>[4x]GAMGSMATRIAILGAGPSGMAQLRAFQSAQEKGAEIPELVCFEKQADWGGQWNYTWRTGLDENGEPVHSSMYRYLWSNGPKECLEFADYTFDEHFGKPIASYPPREVLWDYIKGRVEKAGVRKYIRFNTAVRHVEFNEDSQTFTVTVQDHTTDTIYSAAFDYVVCCTGHFSTPYVPEFEGFEKFGGRILHAHDFRDALEFKDKTVLLVGSSYSAEDIGSQCYKYGAKKLISC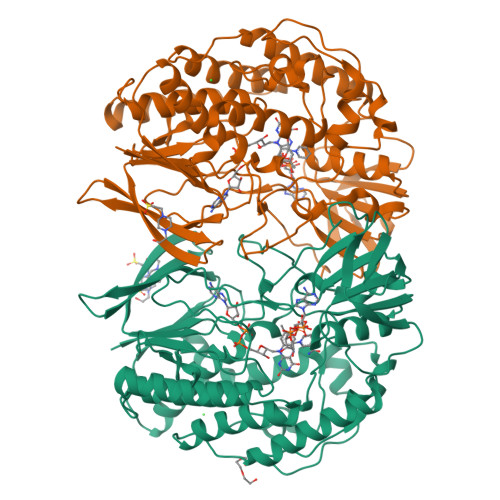YRTAPMGYKWPENWDERPNLVRVDTENAYFADGSSEKVDAIILCTGYIHHFPFLNDDLRLVTNNRLWPLNLYKGVVWEDNPKFFYIGMQDQWYSFNMFDAQAWYARDVIMGRLPLPSKEEMKADSMAWREKELTLVTAEEMYTYQGDYIQNLIDMTDYPSFDIPATNKTFLEWKHHKKENIMTFRDHSYRSLMTGTMAPKHHTPWIDALDDSLEAYLSDKSEIPVAKEA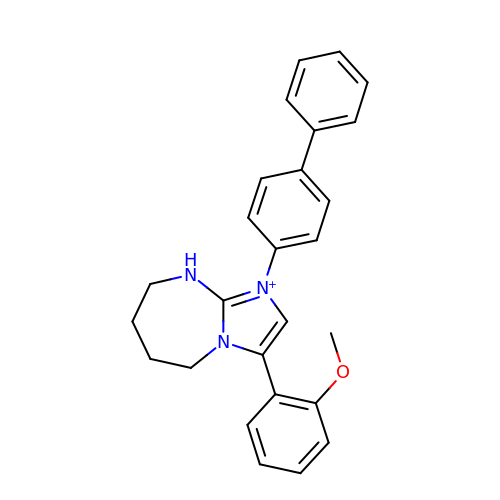3-(2-methoxyphenyl)-1-(4-phenylphenyl)-6,7,8,9-tetrahydro-5~{H}-imidazo[1,2-a][1,3]diazepine | C26 H26 N3 O | HGDBKVRVNGXGJR-UHFFFAOYSA-O> DLDTHFTQYKLARPYIADCPNCGHSRCDSPIAIEEVRGDAHAGVIRIQTSAMFGLKTDGVDLAYMSFMNGKTQKSIKIDNLHVRTSAPCSLVSHHGYYILAQCPPGDTVTVGFHDGPNRHTCTVAHKVEFRPVGREKYRHPPEHGVELPCNRYTHKRADQGHYVEMHQPGLVADHSLLSIHSAKVKITVPSGAQVKYYCKCPDVREGITSSDHTTTCTDVKQCRAYLID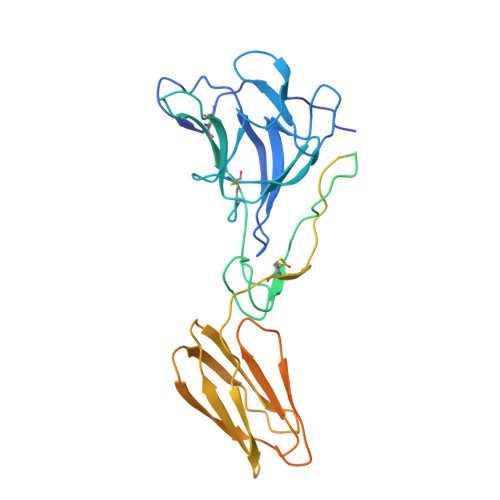NKKWVYNSGRLPRGEGDTFKGKLHVPFVPVKAKCIATLAPEPLVEHKHRTLILHLHPDHPTLLTTRSLGSDANPTRQWIERPTTVNFTVTGEGLEYTWGNHPPKRVWAQESGEGNPHGWPHEVVVYYYNRYPLTTIIGLCTCVAIIMVSCVTSVWLLCRTRNLCITPYKLAPNAQVPILLALLCCIKPTRA> MSQSLEEKSVQERTRIKNSRYESGVIPYAKMGYWNPDYQVKDTDVLALFRVTPQPGVDPIEAAAAVAGESSTATWTVVWTDLLTAADLYRAKAYKVDQVPNNPEQYFAYIAYELDLFEEGSIANLTASIIGNVFGFKAVKALRLEDMRLPFAYIKTFQGPATGVILERERLDKFGRPLLGCTTKPKLGLSGKNYGRVVYEALKGGLDFVKDDENINSQPFMRWRERYLFVMEAVNKAAAATGEVKGHYLNVTAATMEEMYARAQLAKELGSVIIMIDLVIGYTAIQTMAKWARDNDMILHLHRAGNSTYSRQKNHGMNFRVICKWMRMAGVDHIHAGTVVGKLEGDPIITRGFYKTLLLPKLERNLQEGLFFDMDWASLRKVMPVASGGIHAGQMHQLIHYLGEDVVLQFGGGTIGHPDGIQSGATANRVALEAMILARNENRDFLTEGPEILREAAKNCGALRTALDLWKDITFNYTSTDTSDFVETPTANI;> MRITQGTFSFLPDLTDEQIKKQIDYMISKKLAIGIEYTN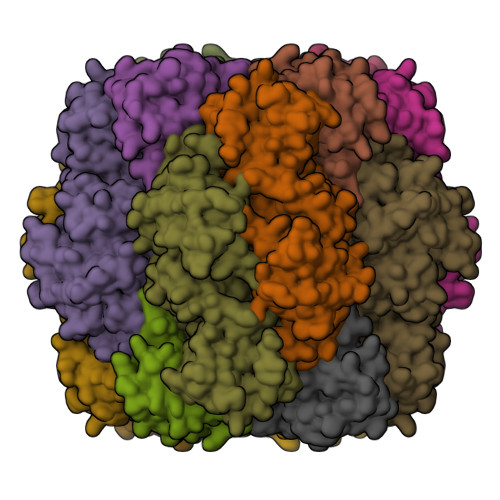DIHPRNSFWEMWGLPLFEVTDPAPVLFEINACRKAKSNFYIKVVGFSSERGIESTIISFIVNRPKHEPGFNLIRQEDKSRSIKYSIQAYETYKPEDQRY> MWNPIVNVDITLNTAGTTREGFGLPLFLASTDNFEERIRGYTSLTEVAEDFDESTAAYKAAKQLWSQTPKVTQLYIGRRTMQYTVSIPDTVAEGSEYSLTVAIGGGVSQPFQYTAKENDTALIVLNEFKSQIEASPTIKDGVNASVTGTGASATMIITKAGDNDFVKVTSITPTTSIAATTADTASAALASIETYSTDWYFISAEDRTQQFVLAMASEIQARKKIFFTANADVKALQGTDLTSATDVPAQLAKSKYTRTVCLWHHTAEFDYPEMAYIAYGAPYDAGSIAWGNAQLTGVAASLQPANQRPLI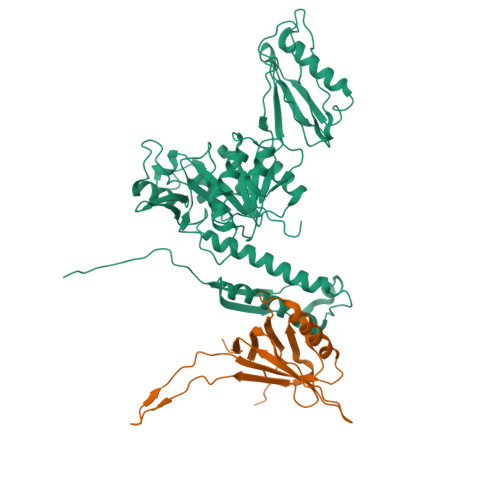SIQKSALDTRSCNFIDLDGGVPVVRRGITSGGEWIDIVRGVDWLESDLKTSLRDLLINQKGGKITYDDTGITRIRQVIETSLQRAVNRKFLSTYTVTVPKASQVALADKKARILKDITFHGILAGAILDVDLKGTVAYE;> MAMYQQYSPKDVVCSWNGIAIEGFAPDSFLRLQRTSPLVTPVVGAGGQVALTRNADKTGTIEIELMQTSLSNQMLSAIQAKQDDMELEEDISSNFVIYDPSGSVLATGINAWLQELPQIELGRDQNSKTWIFGCEKLDYTSTIPASSV>STLH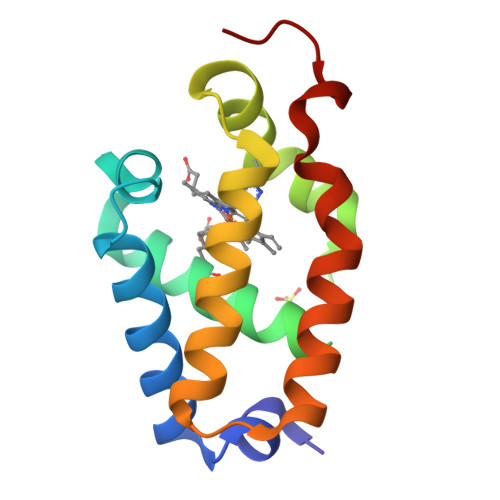AKLGGAAAVAATVDVFYKKLMNDPDLEPFFRGVDMVTLIAKQNRFLAYAFGATTHYHGKDIVMGHAHLIINRGLNLTHFDKVAGHFVDSLKEMGVGQELIDEAAGVLIGVRPLFDPERYKGKVD[2x]>[3x]SREFDFFTYETPKVIVVKSWTIGIINRVVQLLIISYFVGWVFLHEKAYQVRDTAIESSVVTKVKGSGLYANRVMDVSDYVTPPQGTSVFVIITKM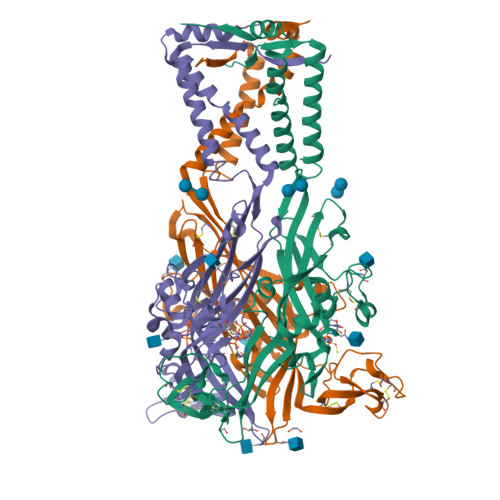IVTENQMQGFCPESEEKYRCVSDSQCGPERLPGGGILTGRCVNYSSVLRTCEIQGWCPTEVDTVETPIMMEAENFTIFIKNSIRFPLFNFEKGNLLPNLTARDMKTCRFHPDKDPFCPILRVGDVVKFAGQDFAKLARTGGVLGIKIGWVCDLDKAWDQCIPKYSFTRLDSVSEKSSVSPGYNFRFAKYYKMENGSEYRTLLKAFGIRFDVLVYGNAGKFNIIPTIISSVAAFTSVGVGTVLCDIILLNFLKGADQYKAKKFEEVNE>[4x]IKPSNILPVTVYDQHGFRILFHFARDPLPGRSDVLVVVVSMLSTAPQPIRNIVFQSAVPKV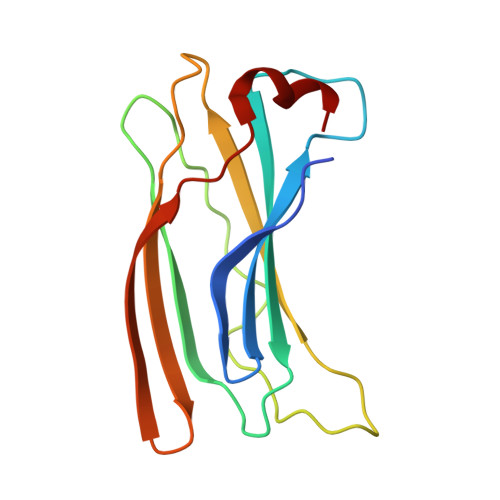MKVKLQPPSGTELPAFNPIVHPSAITQVLLLANPQKEKVRLRYKLTFTMGDQTYNEMGDVDQFPPPETWGSL> SNAMFAPQGLAQFIKVNVTLENGEPVFIYTDANGQVCQGDITVTQAGTITYLLNDQTLKGLKFVGVGFVT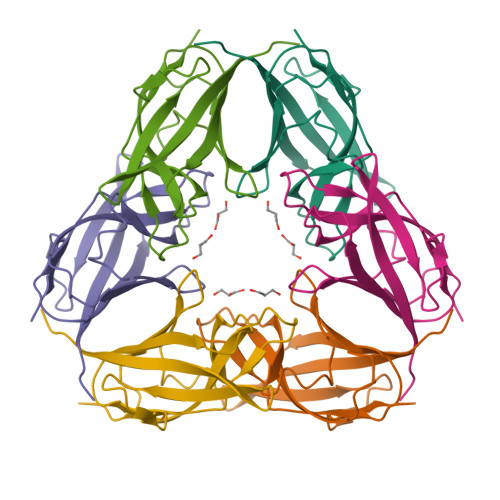PFDGIIDAVTISSDGMLVQLVDLDKTPGTTKFQFVLSNTANTLLVLSPAPQIINRPQN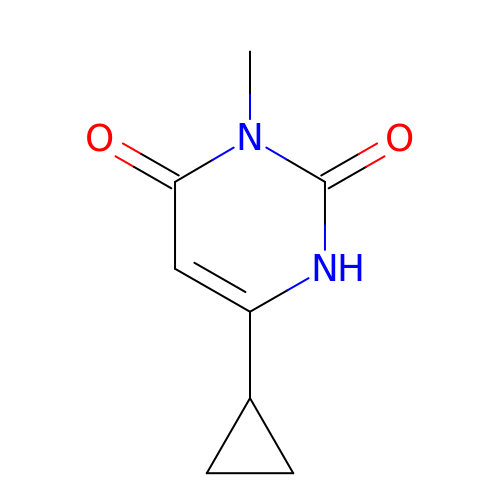6-cyclopropyl-3-methyl-1H-pyrimidine-2,4-dione | C8 H10 N2 O2 | SJCKLNPJUZKFGN-UHFFFAOYSA-N>MRLSWVIGGAQGTGIDTAANIFGNAVASAGYYIYGNREYYSNIKGRHSYFSLTISDKRVRSNTQKIDILVSFDAETVFQHFYDVKDILIYNKAVETTKIDAVQSMEPELAERIKDFLTKQGYETTVKGALEYASKNNVTLIPVNYDEIAKKVADEMKVPLSVTERVKNIVGITISYKLLGLDVNYLIEAINSTFKQDLYRKMNELAVKDSYDIVESRYNLKPSSKERRRFWLDGNTAVAIGKIYGGVRFQSYYPITPASDESVYIEAHQDVLMEDPITGDKKKGTIVVVQAEDELAAINMAIGAALTGVRAATATSGPGFSLMVEGLGWAGMNEVPVVITYYIRGGPSTGLPTRTAQSDLIFPIFAGHGEFPKIVLASGDHAEAFKDAIWALNLAEKYQTPVIHLVEKTLANSYSTIPYEELELDKLKAERGKIVESGDISYKRFKFTEDGISPRAFLGKATMYYTGDEHNEEGHISEDVVNRTMMYEKRMKKLEVADKEIPEESRVKIYGDLNSRNLIITWGSPTGVLRDILEESNFDFTLLQIRMFSPFPKNLVSKLMEGRDKIITVEGNYLAQTSLLVKMYTGKDVTNSILKWNGRPFLRDELEEALIKVIKDGEKRVVLNGGI[2x];>MAAFTPQWNDWCPGCGNFGILNAEQQAIVELGVDTKNVVVVSGIGCSGKIPHFFRTPISGVHTLHGRAIAFATGIKLSNPDLVVIVNGGDGDLLGIGAGHFVAAGRRNVDMVVILHDNGVYGLTKGQASPTLKRGEKPKSLPRPNINDAVNPIALAISSGYTFVARGYAYDVKHLKELIKSAIKHKGLALIDVLQPCPTYNDINTKEWYDKRIYKLDTLPDWDPVVKKPEEVNEKIKRAIDKSLEWGDRIPIGIFYQNELVPSYEERIKANSPAYLDYTPAKQLIEKEGKLTTIIDPLLKEREVD[2x]

In archaea, early branching bacteria, and amitochondrial eukaryotes, the reactions are catalyzed by a much simpler enzyme, 2-oxoacid:ferredoxin oxidoreductase (OFOR). In this study, we report the crystal structures of StOFOR1 and its paralog StOFOR2 (STK_24350 and STK_24330), providing insights into the substrate recognition and reaction mechanism of the (ab)2 type OFORs from extremophilic archaea and bacteria. StOFOR2 and StOFOR1 possess domains III (1a–228a), I (228a–500a), and II (500a–627/628a) of the a-subunit and domain VI (1b–305b) of b-subunit but lack domains IV, V, and VII. The TPP molecules of StOFORs accompany a Mg2+ ion around their pyrophosphate group and are buried at the interface between the a-subunits and b-subunits.

We have been investigating the function of an (ab)2 type OFOR from the hyperthermophilic archaeon Sulfolobus tokodaii strain 7 (StOFOR1), which is composed of a 70 kDa a-subunit (STK_23000, corresponding to fusion domains III-I-II) and a 34 kDa b-subunit (STK_22980, corresponding to domain VI). StOFOR1 is one of the simplest versions of OFORs because it lacks the intramolecular Fd-like domain (domain V), providing a good model system for studying the molecular mechanism of this class of enzymes. StOFOR1 shows broad substrate specificity toward 2-oxoacids, such as pyruvate, 2-oxobutyrate, and 2-oxoglutarate, suggesting that it has multiple roles in glycolysis, gluconeogenesis, the tricarboxylic acid cycle, and amino acid metabolism. The crystals of StOFOR1 grew in solutions containing PEG3350, and we could collect a 2.5 Å resolution data set. However, the very low reproducibility of single crystal formation prevented phase determination and further crystallographic analyses. The StOFOR1 structure was solved by molecular replacement using the StOFOR2 structure as a search model. Superimposition of the StOFOR1 and StOFOR2 structures indicates that they have almost identical active sites. The methyl group of pyruvate in StOFOR2 and the propyl group of 1-hydroxypropyl-TPP in StOFOR1 are surrounded by Ser41a, Thr349a, Asp468a’ (the prime mark indicates that the residue comes from the other protomer), Lys49b and Leu123b. In StOFOR1, mutations at Lys49b and Leu123b, which correspond to Ile843 and Asn996 in DaPFOR, affected the substrate specificity. The K49bR and L123bN mutants exhibited strong preferences for pyruvate and 2-oxoglutarate, respectively.>SGRPMDNEEWFPLKQTHYPPPTIPSMKTGHPTGPISIGHIIPDLRHLDNVINCKGFEPFPPNMDVFTAHYEQCHFGDHLNSEFVVQAGLHHTNITSDRWEYDSVVEYAVYPTRQYIDRLLESKEVRQYIQASAALLGGWCVYMVTGIMVARGGGRNVTSEEKGAGVSGPEVGWDTKTKTKVNAHHTTDFVCAIRLVKIAKSGLRSSW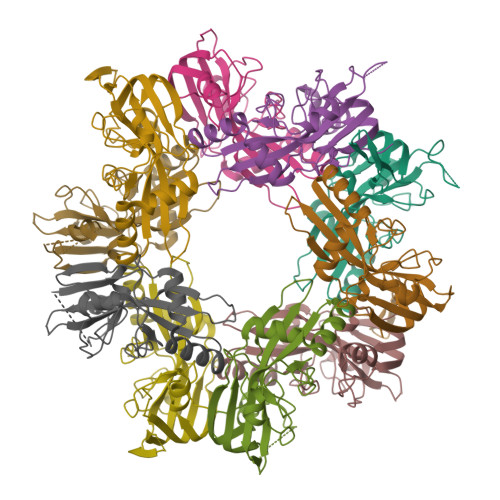TMKKVTREF[10x]(1S,2R,5R,8R,8aR)-5-[2-(4-tert-butylphenyl)ethyl]octahydroindolizine-1,2,8-triol 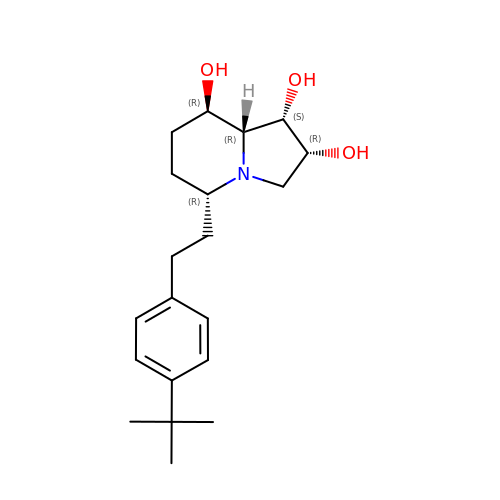| C20 H31 N O3 | QXPSLCODOUKVQZ-FVVUREQNSA-N> SALQDLLRTLKSPSSPQQ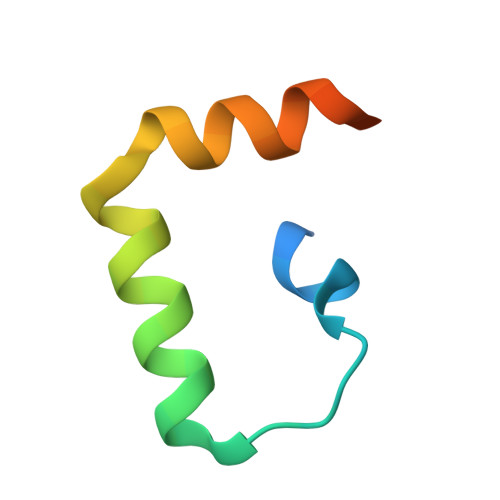QQQVLNILKSNPQLMAAFIKQRTAKYVAN> MGHHHHHHSHMSYARVRAVVMTRDDSSGGWLPLGGSGLSSVT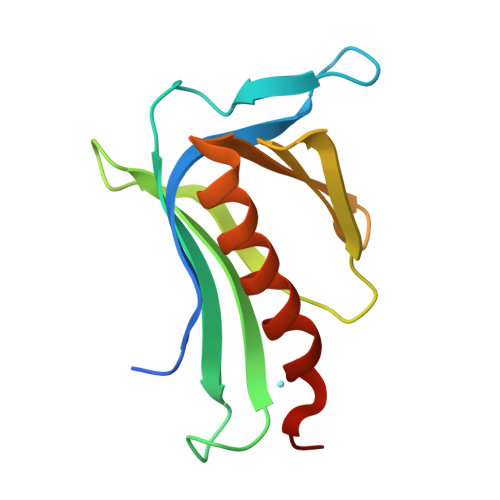VFKVPHQEENGCADFFIRGERLRDKMVVLECMLKKDLIYNKVTPTFHHWKIDDKKFGLTFQSPADARAFDRGIRRAIEDISQGCPESK>GIHHVSIKDVLSKYVQLLPNGSSEFRVVKEKDGSSEILTENQVTFDTKTTSEGLVEVTAKFSPNYSLEDGARYVLKFTVTSSQEALDAIAGDKKLEAGDAEGSDVNKLYSNKGASVTYSYGIGNSQTKTKEYSDNPTFKPSDPLTVPVEVEWQGVTGARTVITADQPSNVELKLVQKNKNGGSDNQDYRKTNVNVSKNVSNETRNFEKVAKGYQYDLIAPDVPAFTKEIKNVGTESNPSFKVIYKQLPSLTIKKVLEAENNLNKEFRIKVKLTSPDSKPLNGTFGEITVVNGEAEIRVEKRKRWRGILSYLPRGTHYKVEEEAASTNGYHVTYENQEGDLN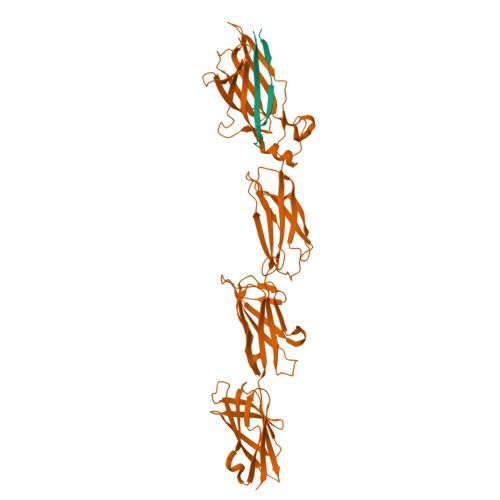KDETSTVTNHKLPSLSVTKKVTGVFANLLKSFKITINIRDAQNSPLNGTYTATVNNKRTPLQFTNGRASIDLNKDQTIKIDGLPLDSHYTVEEETNSSRGYQVSYENQEGKLDGDKSATVTNNKN[2x];>[2x]EPQTTLHKTITPISGQDDKYELSLDITSKL>[2x]MSDQGGGDSTQTAAPVTAPGGAPEPASRPGRSGLGEPSAETIRTGGEEVFAALAERYRHELRVHLYRMLGSFTDAEDLVQETLLKAWRRRETFEGRAGFRAWLYRIATNTALDFLGGPARNREVALAVDSAGSPVSSALAEVSWLQPYPD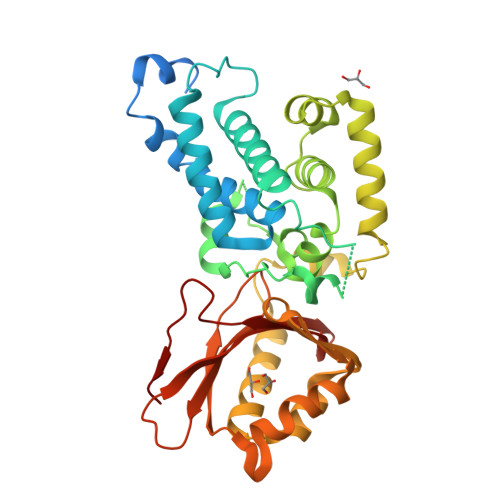RLLDLAAPGTGEPHTAAIARETVELAFLAVIQHLPPRQRAVLILRDIAGWSAQETADALDMTVASVKSALQRARTTLRGRLPERRSEWGAATEPSAAERSLLRRYMAASRDADLSALALLLREDARQAMPPHRLVFDGRDAILDLWRPVLEGDTAWGEWRSVPYAVNRQPAAVSYVRRAGETLFTAVNVDVLTVVDGLIAEITTFDPGLLPGIAPTLAE Bacteriophage E217 infects Pseudomonas aeruginosa and is part of an experimental phage cocktail developed to eradicate P. aeruginosa infections in Galleria mellonella (wax moth) larvae and vertebrate models. E217 is a PB1-like Myoviridae of the Pbunavirus genus characterized by a ~66.2 kbp genome, significantly smaller than the classical enterobacteria phage T4 (~169 kbp). Here, we describe the structure of the whole E217 virion before and after DNA ejection at 3.1 Å and 4.5 Å resolution, respectively, determined using cryogenic electron microscopy (cryo-EM). We identify and build de novo structures for 19 unique E217 gene products, resolve the tail genome-ejection machine in both extended and contracted states, and decipher the complete architecture of the baseplate formed by 66 polypeptide chains.

The baseplate assembles at the tip of the tail apparatus, breaking the repetitive symmetry of the tail tube and sheath protein, creating a unique tip for host attachment, cell adsorption, and genome ejection. The first subunit, gp33, binds the C-terminal ~40 amino acids of gp37 and gp38 that extend outward, while gp34 binds the β-sheet ridge formed by gp37/gp38, generating a hexameric ring above gp33. Notably, both gp33 and gp34 form hexameric assemblies that lack intra-subunit contacts suggesting these proteins are adaptors instead of discrete structural components of the baseplate. The baseplate nut provides an anchoring site for tail fibers, which had poor density in the cryo-EM reconstruction of the extended tail. The baseplate nut assembles outside the cap like a crown and remains bound to the sheath after contraction.

>[6x]MISQSRYIRIISGVGAAAPVAGRKLILRVMTTNNVIPPGIVIEFDNANAVLSYFGAQSEEYQRAAAYFKFISKSVNSPSSISFARWVNTAIAPMVVGDNLPKTIADFAGFSAGVLTIMVGAAEQNITAIDTSAATSMDNVASIIQTEIRKNADPQLAQATVTWNQNTNQFTLVGATIGTGVLAVAKSADPQDMSTALGWSTSNVVNVAGQSADLPDAAVAKSTNVSNNFGSFLFAGAPLDNDQIKAVSAWNAAQNNQFIYTVATSLANLGTLFTLVNGNAGTALNVLSATAANDFVEQCPSEILAATNYDEPGASQNYMYYQFPGRNITVSDDTVANTVDKSRGNYIGVTQANGQQLAFYQRGILCGGPTDAVDMNVYANEIWLKSAIAQALLDLFLNVNAVPASSTGEAMTLAVLQPVLDKATANGTFTYGKEISAVQQQYITQVTGDRRAWRQVQTLGYWINITFSSYTNSNTGLTEWKANYTLIYSKGDAIRFVEGSDVMI;>KIPLTAVPNQAISFNAGSSYWKIRLYQNMDMMNADISRDGVIVCHGVRCFGGIPLLQYSHQYRPDYGNFVFDRDADWTLFGDGINLFYLDGAEFAEYQALAT[6x];>[6x]STSTIRTGTNNDILLDDNGNMVILRDVEACAQDVRAAMLMRTGENIFDVNSGVGYFEYIFSPQKSYDDARKSIADAILSSPDVTGIEQLDIDITGEVFGVDAKVITIH;>[6x]MINVSGFGTGIVIVSASSFPMGFSLSKFADDESPISSKELEPFGYEMLYDGGLFAFDKAAPLEVSVSVIAGSEDDINLRILLNSKKGSFRFLPGIIPDMTTLVATLPDGGRTVLSNGTILKGPAIDTIQNTGRRKGNTYTFVFGSYLGAQTA;>MANYNYIVDTGVIVADTADVLSDVEAEFRAALGANINLAASTPQGSLVAAEAIARSSVMRNEARIANTINPNVSFGTFLDAICALMGIERGSDLSTFGYGVQVTGRSQTRISTGSRVQTPAGAIFTVMSDVTIPAGGVATIDIKSQEYGNIPLPVGNLIIIDGTIGWSGAKVIASTRVDPGSRQMSDAELKNARVNRLAIQGRNSTMAIKAYVSAVPNVTSVNVIENNTGAVQVVNGVSFTLPYAVWVCVAGNPDKQAVADALWAAHNGGTPWDYGATNNGVPVDGPNGVPVRDPASGRKYVVKWTTPIMYDGYVNVTVQQGSSSVAPEAIQNAVVNYAQGKVEGEEGLVVGASLSAFEVAGAIAREIPGIYIKLCQVACVAAGSPAPAPGDFTSEYVMSAFGQATISVGNVRVTFV[6x];>LPAYNSDIQQALKWLHNQAPGITGLIQRKAQWYDRFSRQFWANWERDVFHLKTANPFGLMVWCIILGTPSKGFGLYPKNSSWAFGRLRQNFIYSGTQVPPPADASPGGNFYGGGNAEILNLDEIRKVLQLRYVALISNGSIAYINRMLRYIFNDDEPWDEATGLYFYLMDSTGENGPVENLAVYRKDWEGMVLLSSSPRTNHVLTSTPASDADWPGVDPAASGIPVTVETASATAPDGSATVCKLTKPAGSTAYVSAPIDGPLGSGSTVTFSFFAKAGSTRFIAIQSAADFPSRADAVFDLDSGNVISDQMLDSSVVSARMIRLENGWWRCVLTTKTVSSSFRAAYVAPAETNFSWIDSNSSAAIDVLIWGAQIELGDTPTGYLKTTGAPVTITDYVLQNAQTGTVKFTQPLPTGVEAYWTGDWKGGTAAEPARFAVGNGTQDTFTLSDPAYIGLPTSGAFKLEYRVGPALNLSPQLINLMNDRAVGIMPTCAGCDVKVI[6x]>MTSHFMLRRALLPLAIAALAGCSLAPTYERPQAPVASHWQAADAEGARAQALDWQTFIVDADLRRAVDTALSNNRSLRQALLDIEAARAQYRIQRADRLPSINANASGNRQRLPADLSQTGRSEVTSNYQVGLGLAEYEVDLFGRVRNLSEAALETYLATEEATRATQISLVAEVIQAYLTRDGALRRMALVEQTLDSRMASLELVSQRRAAGAATALDYQEAVGLAEQARAERESTERQLRQADNALVLLLGTPDAARLLPATPRDDLMVLQDIAPGTSSELIERRPDILASEHRLKARNADIGAARAAFFPRISLTGSVGSSSAELSGLFDGGSRAWSFAPTLSLPIFAGGRNRANLDLAEVRQDAAVADYEGTIQTAFREVADALAATDTLRREEAARQALAGSSEAAMALAKARYEGGVDDYLRYLDAQRSTFSNQTTLIQISTERQIALVDLFRSLGGGWGQTEPMAGIGAEHHHHHH[3x];>MNKFREWITFSVISCLVAVTLVGCDKPEEQREEAPAREVDVLSVKTEPFTVFAELPGRIEPVRVAEVRARVAGIVLKRTFEEGADVKAGDVLFQIDPAPFKAALSRAQGELARAEAQLFQAQAMVRRYEPLVKIDAVSQQDFDNAMAALQSAQADKRSAQANVETARLDLGYAEVRAPIAGRIGRAQVTEGALVGQGEATLLARIQQLDPVYADFTQPAADALRLRAAIAEGKVAGASDQPLSLRVDGTDIERKGTLLFTDISVDRSTGQIALRGQFDNPEGVLLPGMYVRVRTPQGLNQNAILVPQRAVQRSADGQASVMLLGEGDTVEVRQVTTGAMQGSRWQISEGLQAGDKVITSSLAAIRPGAKVIPREQGAAEKAPQSQAQWSHPQFEK[6x];>MPLFFIRRPNFAWVVALFISLGGLLVIPFLPVAQYPNVAPPQITVTATYPGASAQVLTDSVTSVIEEELNGAKNLLYFESTSNANGIAEITVTFQPGTDPELAQVDVQNRLKKAEARMPQAVLTLGIQTEQATAGFLLIYSLRYKDGDKNANTTALADYAVRNVNNEIRRLPGVGKLQFFDSEAAMRVWIDPQKLVGYGLSIDDVNNAIRTQNVQVPAGAFGSTPGSSEQELTATLTVKGTLDNPEEFAAIVLRANQDGSRLTLGDVARIEVGSQDYNFGSRQDGKPAVAAAVQLSPGANAIQTAEAVKQRLTELSANFPDNVEFSVPYDTSRFVDVAIDKVIMTLIEAMVLVFLVMFLFLQNVRYTLIPSIVVPVCLLGTLTFMYLLGFSVNMMTMFGMVLAIGILVDDAIVVVENVERIMAEEGLAPVPATIKAMGQVSGAIIGITLVLSAVFLPLAFMAGSVGVIYQQFSLSLAVSILFSGFLALTFTPALCATLLKPIPVGHHEKTGFFGWFNRKFTSLTSRYTKLNDKLVPRAGRVMFIYLGVVVLMGFLYMRLPESFVPVEDQGYMIVDIQLPPGATRERTSAAGGELESFLMAREAVQTTFLVLGFSFSGMGENAAIAFPLLKDWSERDSSQSPEAESAAVNQHFANLDDGAIMAVPPPPVEGLGNSGGFALRLQDRAGLGRDALLAARDEVLGKVNGNPKFLYAMMEGLAEAPQLRLVIDREQARTLGVSFEAISSALSTAFGSSVINDFANAGRQQRVVVQAEQAERMTPESVLRLHVPNDSGSLVPLSAFVTTSWEEGPVQVARYNGYPSIRIAGDAAPGVSTGEAMLELERIAAELPEGIGYEWTGLSYQERVASGQATMLFALAITVVFLLLVALYESWAIPLTVMLIVPVGALGAVLAVTAIGLPNDVYFKVGLITVIGLAAKNAILIVEFA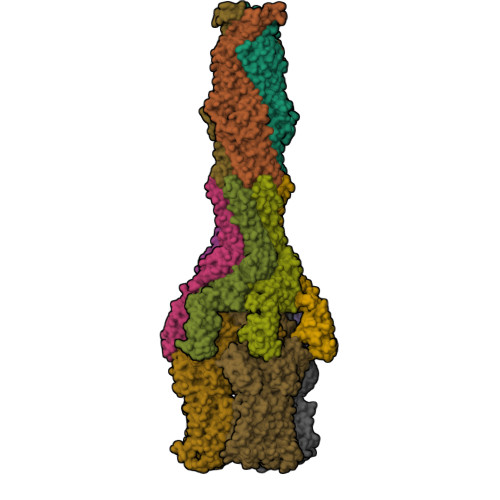KDLWEDGYSLRDAAVEAARLRFRPIIMTSMAFMLGVVPLAIATGAGAASQRALGTGVLGGMLSATMLGVIFVPIFFVWVLSLLRTKPQQTDNHPLHKAE[3x]> MHHHHHHHAVRASEISRVYEAYPEKKATLYFLVLGFLALIVGSLFGPFQALNYGNVDAYPLLKRLLPFVQSYYQGLTLHGVLNAIVFTQLFAQAIMVYLPARELNMRPNMGLMWLSWWMAFIGLVVFALPLLANEATVLYTFYPPLKGHWAFYLGASVFVLSTWVSIYIVLDLWRRWKAANPGKVTPLVTYMAVVFWLMWFLASLGLVLEAVLFLLPWSFGLVEGVDPLVARTLFWWTGHPIAYFWLLPAYAIIYTILPKQAGGKLVSDPMARLAFLLFLLL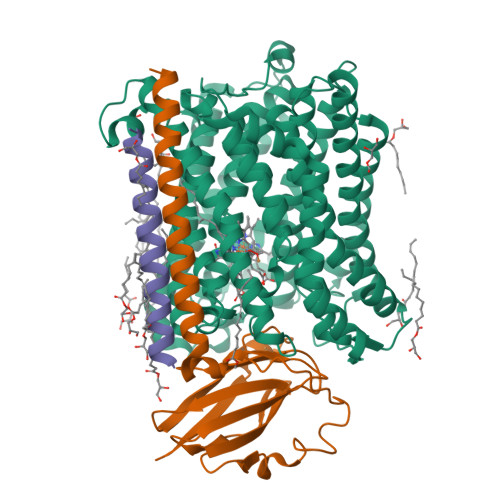STPVGFHHQFADPGIDPTWKMIHSVLTLFVAVPSLMTAFTVAASLEFAGRLRGGRGLFGWIRALPWDNPAFVAPVLGLLGFIPGGAGGIVNASFTLDYVVHNTAWVPGHFHLQVASLVTLTAMGSLYWLLPNLTGKPISDAQRRLGLAVVWLWFLGMMIMAVGLHWAGLLNVPRRAYIAQVPDAYPHAAVPMVFNVLAGIVLLVALLLFIYGLFSVLLSRERKPELAEAPLPFAEVISGPEDRRLVLAMDRIGFWFAVAAILVVLAYGPTLVQLFGHLNPVPGWRLW;> MVDEHKAHKAILAYEKGWLAFSLAMLFVFIALIAYTLATHTAGVIPAGKLERVDPTTVRQEGPWADPAQAVVQTGPNQYTVYVLAFAFGYQPNPIEVPQGAEIVFKITSPDVIHGFHVEGTNINVEVLPGEVSTVRYTFKRPGEYRIICNQYCGLGHQNMFGTIVVKE;> MEEKPKGALAVILVLTLTILVFWLGVYAVFFARG> VVGGHPGNSPWTVSLRNRQGQHFCGGSLVKEQWILTARQCFSSCHMPLTGYEVWLGTLFQNPQHGEPSLQRVPVAKMVCGPSGSQLVLLKLERSVTLNQRVALICLPPEWYVVPPGTKCEIAGWGETKGTGNDTVLNVALLNVISNQECNIKHRGRVRE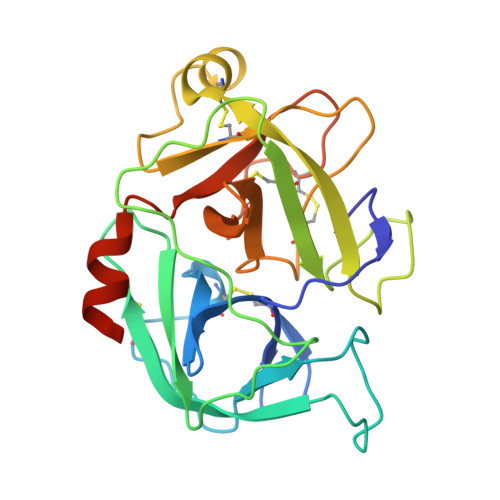SEMCTEGLLAPVGACEGDYGGPLACFTHNSWVLEGIIIPNRVCARSRWPAVFTRVSVFVDWIHKVMRLGHHHHHH>TADELVFFVNGKKVVEKNADPETTLLAYLRRKLGLRGTKLGCGEGGCGACTVMLSKYDRLQDKIIHFSANACLAPICTLHHVAVTTVEGIGSTKTRLHPVQERIAKSHGSQCGFCTPGIVMSMYTLLRNQPEPTVEEIEDAFQGNLCRCTGYRPILQGFRTFAK[2x];>LFNPEEFMPLDPTQEPIFPPELLRLKDVPPKQLRFEGERVTWIQASTLKELLDLKAQHPEAKLVVGNTEIGIEMKFKNQLFPMIICPAWIPELNAVEHGPEGISFGAACALSSVEKTLLEAVAKLPTQKTEVFRGVLEQLRWFAGKQVKSVASLGGNIITASPISDLNPVFMASGTKLTIVSRGTRRTVPMDHTFFPSYRKTLLGPEEILLSIEIPYSREDEFFSAFKQASRREDDIAKVTCGMRVLFQPGSMQVKELALCYGGMADRTISALKTTQKQLSKFWNEKLLQDVCAGLAEELSLSPDAPGGMIEFRRTLTLSFFFKFYLTVLKKLG[2x];>[2x]DTVGRPLPHLAAAMQASGEAVYCDDIPRYENELFLRLVTSTRAHAKIKSIDVSEAQKVPGFVCFLSADDIPGSNETGLFNDETVFAKDTVTCVGHIIGAVVADTPEHAERAAHVVKVTYEDLPAIITIEDAIKNNSFYGSELKIEKGDLKKGFSEADNVVSGELYIGGQDHFYLETHCTIAIPKGEEGEMELFVSTQNAMKTQSFVAKMLGVPVNRILVRVKRMGGGFGGKETRSTLVSVAVALAAYKTGHPVRCMLDRNEDMLITGGRHPFLARYKVGFMKTGTIVALEVDHYSNAGNSRDLSHSIMERALFHMDNCYKIPNIRGTGRLCKTNLSSNTAFRGFGGPQALFIAENWMSEVAVTCGLPAEEVRWKNMYKEGDLTHFNQRLEGFSVPRCWDECLKSSQYYARKSEVDKFNKENCWKKRGLCIIPTKFGISFTVPFLNQAGALIHVYTDGSVLVSHGGTEMGQGLHTKMVQVASKALKIPISKIYISETSTNTVPNSSPTAASVSTDIYGQAVYEACQTILKRLEPFKKKNPDGSWEDWVMAAYQDRVSLSTTGFYRTPN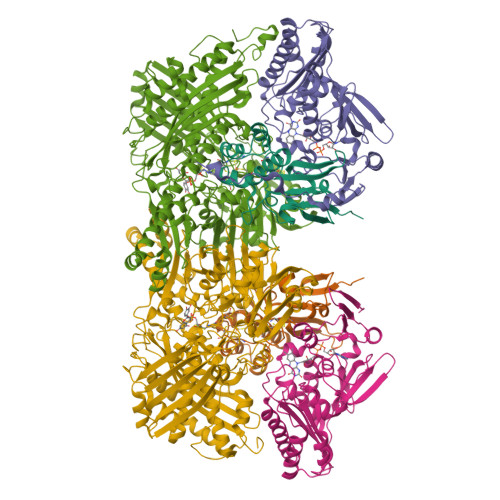LGYSFETNSGNAFHYFTYGVACSEVEIDCLTGDHKNLRTDIVMDVGSSLNPAIDIGQVEGAFVQGLGLFTLEELHYSPEGSLHTRGPSTYKIPAFGSIPTEFRVSLLRDCPNKKAIYASKAVGEPPLFLGASVFFAIKDAIRAARAQHTNNNTKELFRLDSPATPEKIRNACVDKFTTLCVTGAPGNCK>[4x]MFFNKKNNQDELKKLAATEAAKSITTEITLGVGTGSTVGFLIEELVNYRDKIKTVVSSSEDSTRKLKALGFDVVDLNYAGEIDLYIDGADECNNHKELIKGGGAALTREKICVA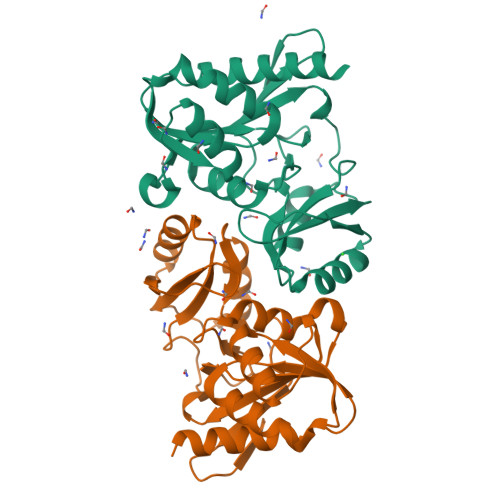AAKKFICIIDESKKVNTLGNFPLPIEVIPMARSYIARQIVKLGGQPVYREQTITDNGNVILDVYNLKIDNPLKLETELNQITGVVTNGIFALKPADTVIMATKDSNIVVL>MAHHHHHHMTGTIGLIWAQTRAGVIGADGAIPWRLPEDQARFKRITMGHTVIMGRKTWESLPGSVRPLPGRPNIVLTRDALFEPDGALAVGSADAALAASDEAPWVIGGGEIYRLFLPLAQRCEVTVVEADVPGDALAPELGE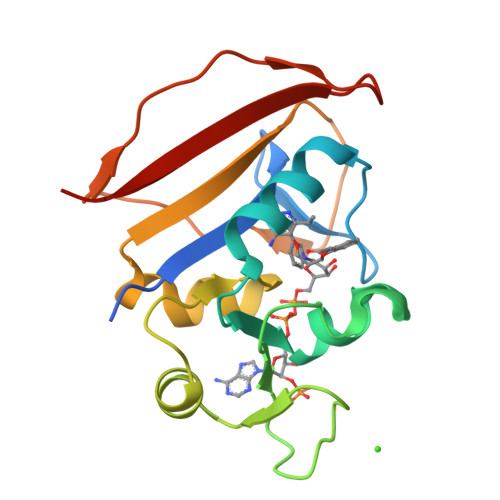GWVVETNDWQTSESGLRYQFLSYRKVDG[7x]> ASMTGWKIHYTSTAHACPYPMAPPNGHVSPVQAKYILKDSFSIFCETGY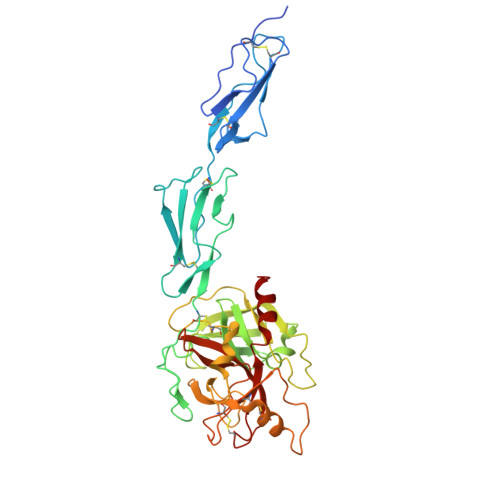ELLQGHLPLKSFTAVCQKDGSWDRPMPACSIVDCGPPDDLPSGRVEYITGPGVTTYKAVIQYSCEETFYTMKVNDGKYVCEADGFWTSSKGEKSLPVCEPVCGLSARTTGGQIYGGQKAKPGDFPWQVLILGGTTAAGALLYDNWVLTAAHAVYEQKHDASALDIRMGTLKRLSPHYTQAWSEAVFIHEGYTHDAGFDNDIALIKLNNKVVINSNITPICLPRKEAESFMRTDDIGTASGWGLTQRGFLARNLMYVDIPIVDHQKCTAAYEKPPYPRGSVTANMLCAGLESGGKDSCRGDSGGALVFLDSETERWFVGGIVSWGSMNCGEAGQYGVYTKVINYIPWIENIISDF>[2x]PTEFLYTSKIAAISWAATGGRQQRVYFQDLNGKIREAQRGGDNPWTGGSSQNVIGEAKLFSPLAAVTWKSAQGIQIRVYCVNKDNILSEFVYDGSKWITGQLGSVGVKVGSNSKLAALQWGGSESAPPNIRVYYQKSNLSGSSIHEYVWSGKWTAGASFGSTAPGTGIGATAIGPGRLRIYYQATDNKIREHCWDSNSWYVGGFSAS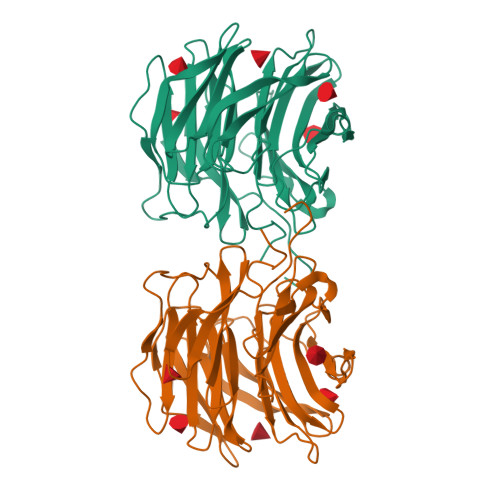ASAGVSIAAISWGSTPNIRVYWQKGREELYEAAYGGSWNTPGQIKDASRPTPSLPDTFIAANSSGNIDISVFFQASGVSLQQWQWISGKGWSIGAVVPTGTPAGW> NEVKYPVVYEIFIRSLYDSDGDGVGDINGVSQKVDYLRKLGIDAVWFMPFNEAVSYHGYDITDYYNVEKDYGTMEDLENMIQVLHENGIKVIMDLVINHTSDEHPWFKDAVENTTSSPYWDYYIMSLEDHSGQDHWHWKINSKGQKVWYFGLFGYNMPDLNHDSQKVREEVKKIVDFWISKGVDGFRIDAAKHIYGWSWDDGIQESAEYFEWFRDYVLSKKPDAILVGEVFSGNTYDLSLYPIPVFNFALMYSIRNYPEGQDGMIENNWVEESFLFLENHDLHRFFSHLQEHYKKFS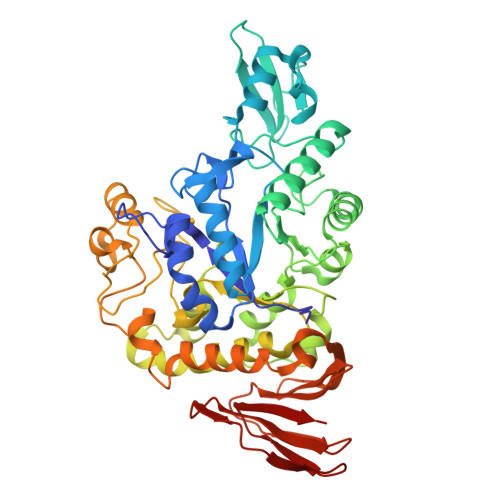ESDYEFIKKRAALWYFLIFTLKGSPVIYYGGEIGTRGFKWHGPVYDEPVREPMQWYASGTGEGQTFWTKEVYKNAGITFGNADVDGCIYDDPYDGFSVEEQENDPKSLLNFIRFILNFRKDHDAILNGDQTIFRDWKNLIAFYRESSNEKLLVVLNPDPVWQNSFTFEENMTMILEVDFENFIWNESNVSFSAGESFTVDPMKAYIFKK> MPDTTPVAATSSAPPTAKDAGAKAPSDFSNPNTAPSLSDLKKVKYVSTVTSVATPAEIEALGKIFTAMGLAANETGPAMWDLARAYADVQSSKSAQLIGATPSNPALSRRALAAQFDRINITPRQFCMYFAKV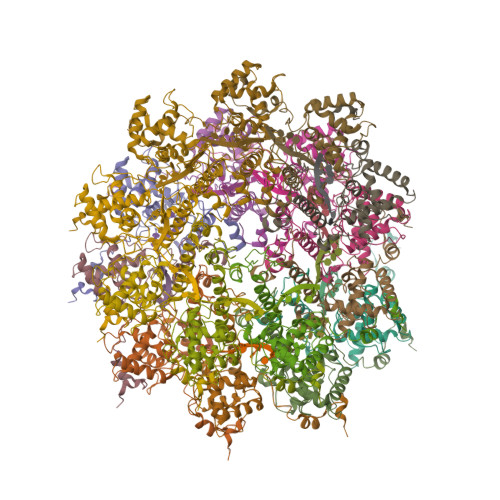VWNILLDSNIPPANWAKLGYQEDTKFAAFDFFDGVTNPASLQPADGLIRQPNEKELAAHSVAKYGALARQKISTGNYITTLGEVTRGHMGGANTMYAIDAPPEL GUANIDINE-3-PROPANOL | C4 H12 N3 O | 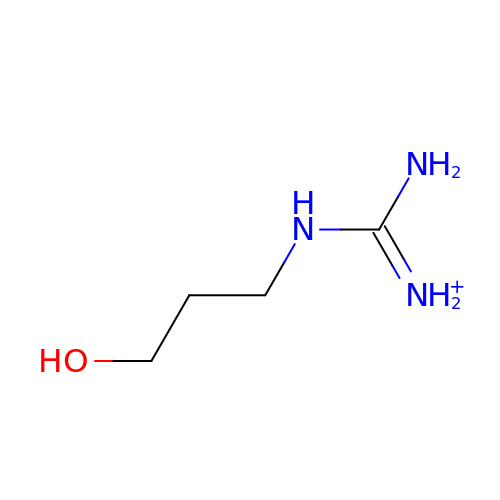JDXXTKLHHZMVIO-UHFFFAOYSA-O>[2x]MHADTATRQHWMSVLAHSQPAELAARLNALNITADYEVIRAAETGLVQIQARMGGTGERFFAGDATLTRAAVRLTDGTLGYSWVQGRDKQHAERCALIDALMQQSRHFQNLSETLIAPLDADRMARIAARQAEVNASRVDFFTMVRGDNA;>MTLETAFMLPVQDAQHSFRRLLKAMSEPGVIVALHQ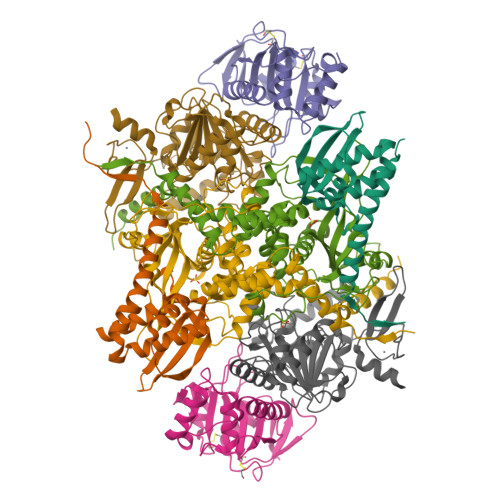LKRGWQPLNIATTSVLLTLADNDTPVWLSTPLNNDIVNQSLRFHTNAPLVSQPEQATFAVTDEAISSEQLNALSTGTAVAPEAGATLILQVASLSGGRMLRLTGAGIAEERMIAPRLPECILHELTERPHPFPLGIDLILTCGERLLAIPRTTHVEVC[2x];>MYVAVKGGEKAIDAAHALQESRRRGDTDLPELSVAQIEQQLNLAVDRVMTEGGIADRELAALALKQASGDNVEAIFLLRAYRTTLAKLAVSEPLDTTGMRLERRISAVYKDIPGGQLLGPTYDYTHRLLDFTLLANGEAPTLTTADSEQQPSPHVFSLLARQGLAKFEEDSGAQPDDITRTPPVYPCSRSSRLQQLMRGDEGYLLALAYSTQRGYGRNHPFAGEIRSGYIDVSIVPEELGFAVNVGELLMTECEMVNGFIDPPGEPPHFTRGYGLVFGMSERKAMAMALVDRALQAPEYGEHATGPAQDEEFVLAHADNVEVAGFVSHLKLPHYVDFQAELELLKRLQQEQNHG[2x];>MANLSGYNFAYLDEQTKRMIRRAILKAVAIPGYQVPFGGREMPMPYGWGTGGIQLTASVIGESDVLKVIDQGADDTTNAVSIRNFFKRVTGVNTTERTDDATVIQTRHRIPETPLTEDQIIIFQVPIPEPLRFIEPRETETRTMHALEEYGVMQVKLYEDIARFGHIATTYAYPVKVNGRYVMDPSPIPKFDNPKMDMMPALQLFGAGREKRIYAVPPFTRVESLDFDDHPFTVQQWDEPCAICGSTHSYLDEVVLDDAGNRMFVCSDTDYCRQQSEAKNQ[2x]> MKIKNITWSFMIALTAVGSGFTSCADQPDKFELASGTPTVYYIRPVDVASKDSLLTSASLQSTICLVGDNLKSIKGILFNDQAAVLNTSYITDHTLIVSVPNEIPSVVTDKMYMITASNDTIPYDFQVTISAPSVVSMSNEWAKAGEEVTITGDYFLDYDNYPLEIKVGKDYTLPREAITSIEK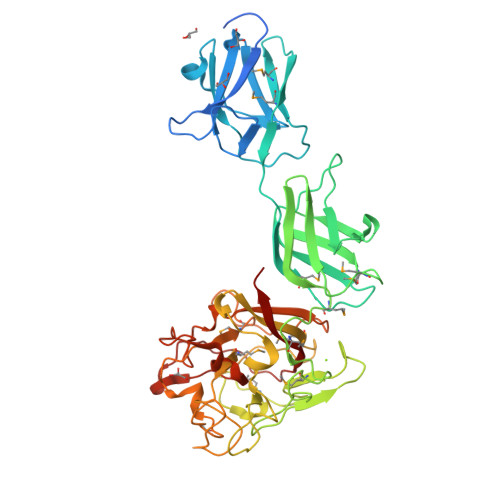TKITFTMPEDMPQHEDIVVSDKYGSTNAPFQYMDNRGMLFDFDTPNSVTNEVLGNSGWHDRIIQSDDTSLSGNYMQIGNTGVTMAANGKWNDEFSFEYWAGNWANPETYASHPRLCDVADFSDWTNKSLKFEMLIPADAGWGAGPMQIIFGSPSQISLGNAGVVDVNGVTLAGCNNTWFHAQNGWGRAIYMPWYSNSSASLYDTGDKWVTVTIPLSDFNLEFDGNSATKSFSSINDFSSLNIFLIKGAYNDKSVLPDGVECTPIIKIDNIRVVPNK> SNAMKDVLAEYASRIVSAEEAVKHIKNGERVALSHAAGVPQSCVDALVQQADLFQNVE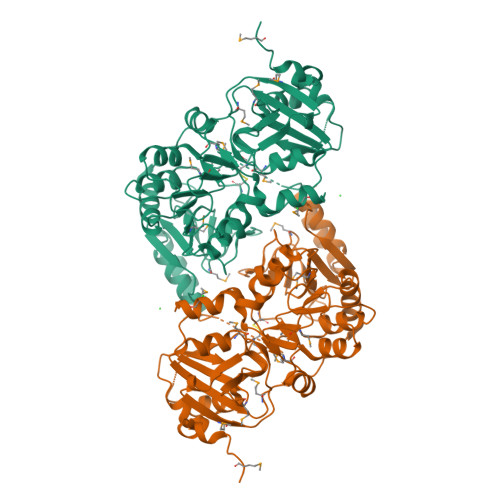IYHMLCLGEGKYMAPEMAPHFRHITNFVGGNSRKAVEENRADFIPVFFYEVPSMIRKDILHIDVAIVQLSMPDENGYCSFGVSCDYSKPAAESAHLVIGEINRQMPYVHGDNLIHISKLDYIVMADYPIYSLAKPKIGEVEEAIGRNCAELIEDGATLQLGIGAIPDAALLFLKDKKDLGIHTEMFSDGVVELVRSGVITGKKKTLHPGKMVATFLMGSEDVYHFIDKNPDVELYPVDYVNDPRVIAQNDNMVSINSCIEIDLMGQVVSECIGSKQFSGTGGQVDYVRGAAWSKNGKSIMAIPSTAKNGTASRIVPIIAEGAAVTTLRNEVDYVVTEYGIAQLKGKSLRQRAEALIAIAHPDFREELTKHLRKRFG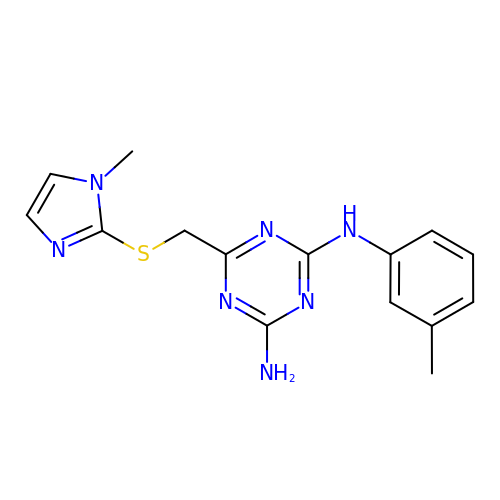6-[(1-methylimidazol-2-yl)sulfanylmethyl]-~{N}4-(3-methylphenyl)-1,3,5-triazine-2,4-diamine | C15 H17 N7 S | AJMVTEFCEYDLAV-UHFFFAOYSA-N>[2x]HLVCPMSKSPYVDPHKSGHEIWEEFSMSFTPAVKEVVEFAKRIPGFRDLSQHDQVNL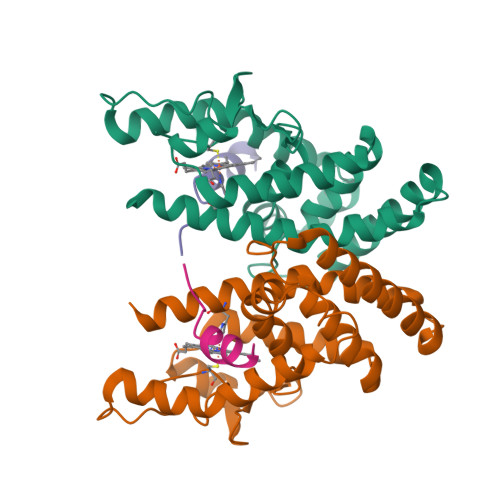LKAGTFEVLMVRFASLFDAKERTVTFLSGKKYSVDDLHSMGAGDLLNSMFEFSEKLNALQLSDEEMSLFTAVVLVSADRSGIENVNSVEALQETLIRALRTLIMKNHPNEASIFTKLLLKLPDLRSLNNMHSEELLAFKVHP;>[2x]RTHRLITLADHICQIITQDFARN> GPLGSMANRDDIDASAVMAAYLAREYAEAVEEQLTPRERDALEALRVSGEEVRSPLLQELSNAGEHRANPENSHIPAALVSALLEAPTSPGRMVTAVELCAQMGRLWTR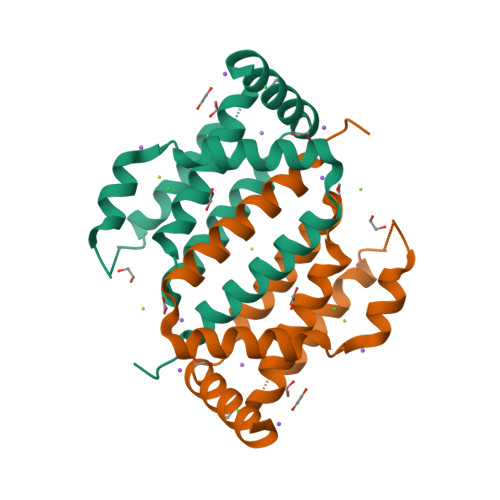GRQLVDFMRLVYVLLDRLPPTADEDLGAWLQAVARVHGT> MSNLPHEPEFEQAYKELASTLENSTLFQKNPEYRKALAVVSVPERVIQFRVVWEDDAGNVQVNRGFRVQFNSALGPYKGGLRFHPSVNLSILKFLGFEQIFKNALTGLNMGGGKGGSDFDPKGKSDNEIRRFCVSFMTELCKHIGADTDVPAGDIGVTGREVGFLFGQYRKIRNQWEGVLTGKGGSWGGSLIRPEATGYGVVYYVEHMIAHATNGQESFKGKRVAISGSGNVAQYAALKVIELGGSVVSLSDSQGSLIINGEGSFTPEEIELIAQTKVERKQLASIVGAAPFSDANKFKYIAGARPWVHVGKVDVALPSATQNEISGEEAQVLINAGCKFIAEGSNMGCTQEAIDTFEAHRTANAGAAAIWYAPGKAANAGGVAVSGLEMAQNSARLSWTSEEVDARLKDIMRDCFKNGLETAQEYATPAEGVLPSLVTGSNIAGFTKVAAAMKDQGD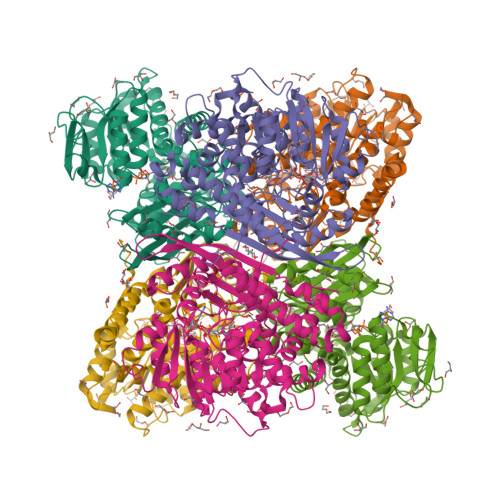WW>[4x]GSHMSLAGKEFKLSNGNKIPAVAFGTGTKYFKRGHNDLDKQLIGTLELALRSGFRHIDGAEIYGTNKEIGIALKNVGLNRKDVFITDKYNSGNH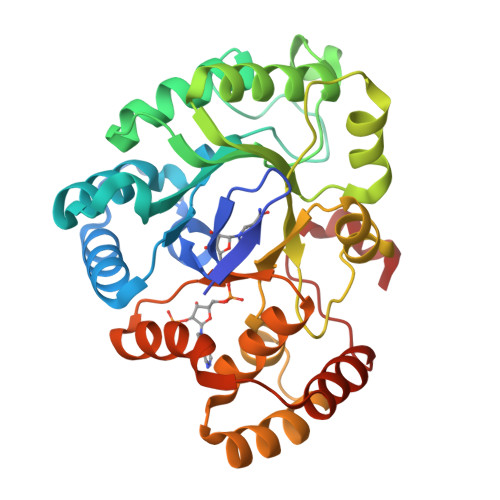TYDGKHSKHQNPYNALKADLEDLGLEYVDLYLIHFPYISEKSHGFDLVEAWRYLERAKNEGLARNIGVSNFTIENLKSILDANTDSIPVVNQIEFSAYLQDQTPGIVEYSQQQGILIEAYGPLGPITQGRPGPLDKVLSKLSEKYKRNEGQILLRWVLQRGILPITTTSKEERINDVLEIFDFELDKEDEDQITKVGKEKTLRQFSKEYSKYD> GPGSMALIERIGKALEPLMLVMGLISPLATMPQLYKLYVSH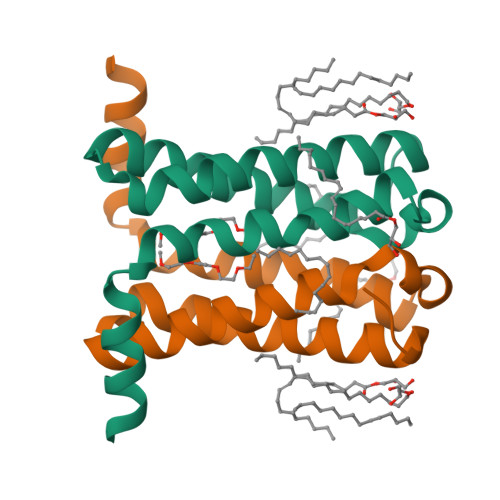SEHALGLSLTTWLLYSFIALLWTIYGIYHKNPTIWVGNCLGFLMYVAMVVGIIAHTGGTY> SNAMSRIIMLIPTGTSVGLTSVSLGVIRAMERKGVRLSVFKPIAQPRTGGDAPDQTTTIVRANSSTTTAAEPLKMSYVEGLLSSNQKDVLMEEIVANYHANTKDAEVVLVEGLVPTRKHQFAQSLNYEIAKTLNAEIVFVMSQGTDTPEQLKERIELTRNSFGGAKNTNITGVIVNKLNAPVDEQGRTRPDLSEIFDDSSKAKVN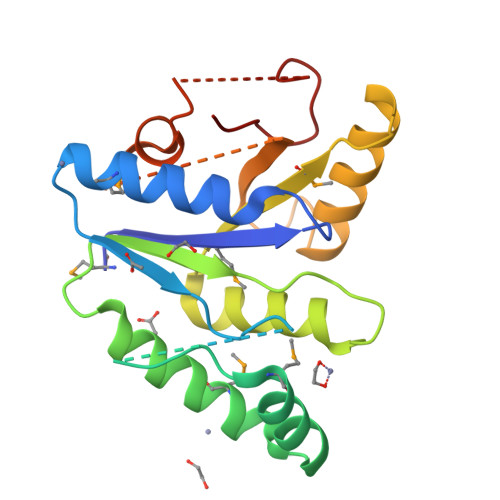NVDPAKLQESSPLPVLGA> MNQNLLVTKRDGSTERINLDKIHRVLDWAAEGLHNVSISQVELRSHIQFYDGIKTSDIHETIIKAAADLISRDAPDYQYLAARLAIFHLRKKAYGQFEPPALYDHVVKMVEMGKYDNHLLEDYTEEEFKQMDTFIDHDRDMTFSYAAVKQLEGKYLVQNRVTGEIYESAQFLYILVAACLFSNYPRETRLQYVKRFYDAVSTFKISLPTPIMSG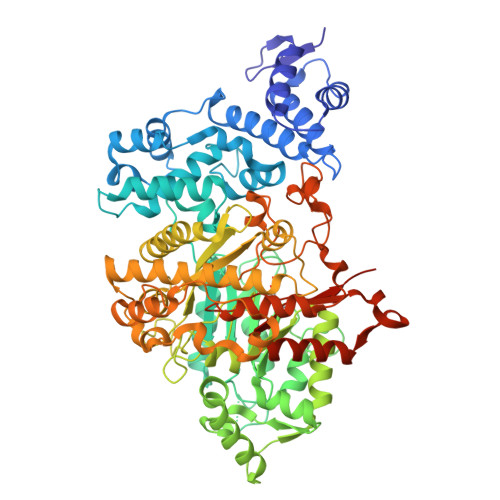VRTPTRQFSSCVLIECGDSLDSINATSSAIVKYVSQRAGIGINAGRIRALGSPIRGGEAFHTGCIPFYKHFQTAVKSCSQGGVRGGAATLFYPMWHLEVESLLVLKNNRGVEGNRVRHMDYGVQINKLMYTRLLKGEDITLFSPSDVPGLYDAFFADQEEFERLYTKYEKDDSIRKQRVKAVELFSLMMQERASTGRIYIQNVDHCNTHSPFDPAIAPVRQSNLALEIALPTKPLNDVNDENGEIALCTLSAFNLGAINNLDELEELAILAVRALDALLDYQDYPIPAAKRGAMGRRTLGIGVINFAYYLAKHGKRYSDGSANNLTHKTFEAIQYYLLKASNELAKEQGACPWFNETTYAKGILPIDTYKKDLDTIANEPLHYDWEALRESIKTHGLRNSTLSALMPSETSSQISNATNGIEPPRGYVSIKASKDGILRQVVPDYEHLHDAYELLWEMPGNDGYLQLVGIMQKFIDQSISANTNYDPSRFPSGKVPMQQLLKDLLTAYKFGVKTLYYQNTRDGAEDAQDDLVPSIQDDGCESGACKI(3S)-5-fluoro-3-hydroxy-1,3-dihydro-2H-indol-2-one | C8 H6 F N O2 | 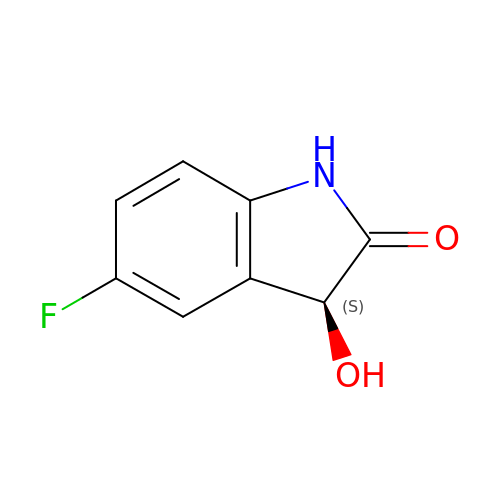XYDTZHMQTYEJQN-ZETCQYMHSA-N6-Azido-L-lysine | C6 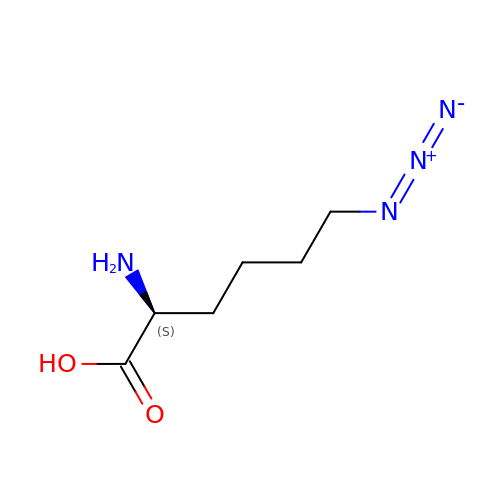H12 N4 O2 | HTFFMYRVHHNNBE-YFKPBYRVSA-N>[4x]GAINKNMKLGQKVLIPVKQFPKFNFVGKLLGPRGNSLKRLQEETLTKMSI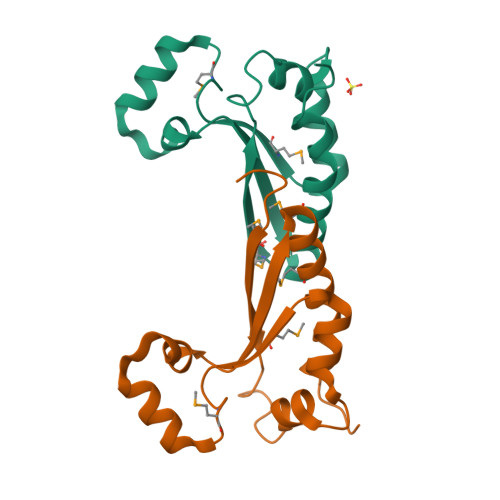LGKGSMRDKAKEEELRKSGEAKYFHLNDDLHVLIEVFAPPAEAYARMGHALEEIKKFLIPDYN2-[4-(aminomethyl)-2-chloro-6-methoxyphenoxy]-N-tert-butylacetamide | C14 H21 Cl N2 O3 | 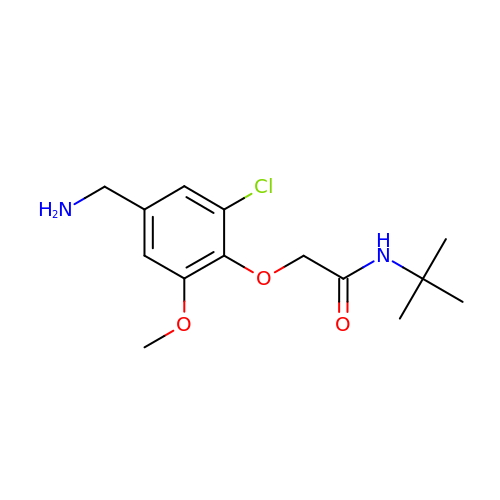HEOFBSUCMHLHRB-UHFFFAOYSA-N>SNAMLLYTKKDDIYSDIVRMILLIKGANAKIVDVSKEENSKHLEELNIITPNGNIPTLSTDDFAVYRLSVIIEAIEDLYPFPPMFPVFPKQRANARILLEYVNKTFLQNIIKLQSPDLDEKQANEIKMLMQRDIISTYKKIVSEREVNAESNPDAQNINVLTLIITFVFYYFI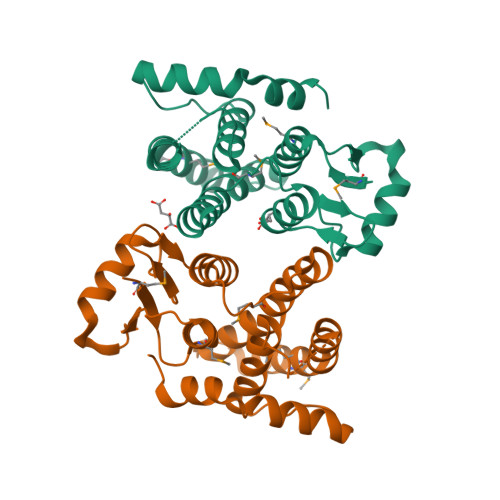KLKISIPTKDKNIIKEIKELLSEPNFIKTIKAKGA[2x]>SATTPPGDLEQPELEARVKEIIEVDGYQFRDLNDNGELDPYEDWRLPTPERVADLVGQMSLVEKSGLMLINTLNAACDPQTGEFGVLPAQADNYINTQHMHRFVFRNVVDVRAEGVECTGTGTPVVSPAEAATFTNAVQEMSEATRLGIPSLFKSNARNHIDPDARVGINEAAGAFSAFPKEAGIAAAALGEQARRTGEATTGDMSVVADFADVMGEEWASIGLRGMYGYMADLSTEPRWYRTHETFTEDAYLAAEIMETLVQTLQGEELTDNGLALSPQTRVALTLKHFPGGGPQELGLDPHYAFGKAQVYPAGRFEEHFLPFQAAIDAGVSSIMPYYGVPVDVPVVGGEPGETYPHTGFAFSDSIVNGLLRDQLGFTGYVNSATGIINDRAWGLEGNTVPERVAAAINGGTDTLSGFSDVSVITDLYEADLISEERIDLAAERLLEPLFDMGLFENPYVDPDVATATVGADDHRAVGLDLQRKSLVLLQNEETDEGPVLPLKEGGDVYILGDFT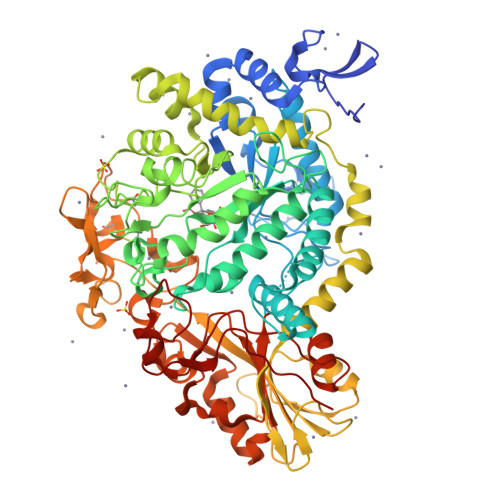EETVESYGYEVTNGNVAEGEERPSAAGSDYVLISMTAKTNAGDYVSDDPSLGLNPDHGTNPSVIIGDDGEPLPGLDGQSLWGAADVCVHKEGHEENPSCTDNRLRFGGAYPWESSILDFTGMEAAESWEVVPSLETIQEVMAEVEDPSKVILHVYFRQPYVLDEESGLRDAGAILAGFGMTDTALMDVLTGAYAPQGKLPFALAGTREAIIEQDSDRPGYDETEDGALYPFGYGLTYEDDTEE[2x]> MNSDEVQLIKKTWEIPVATPTDSGAAILTQFFNRFPSNLEKFPFRDVPLEELSGNARFRAHAGRIIRVFDESIQVLGQDGDLEKLDEIWTKIAVSHIPRTVSKESYNQLKGVILDVLTAASSLDESQAATWAKLVD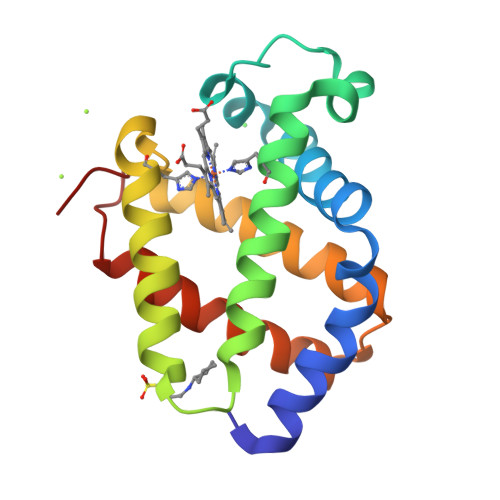HVYAIIFKAIDDDGNAK>[4x]HMSVNKVTCLVCRKGDNDEFLLLCDGCDRGCHIYCHRPKMEAVPEGDWFCTVCLAQQV;>ARTKQTARKS[2x]

The plant homeodomain (PHD) finger is one of the largest families of epigenetic reader domains present in chromatin-related proteins, with over 170 PHD fingers identified in the human genome. Members of the BAZ family of proteins, which includes BAZ1A, also known as Acf1, BAZ1B, also known as Wstf, BAZ2A, also known as TIP5 (TTF-I/interacting protein 5), and BAZ2B, are all characterized by the presence of a PHD–BRD tandem module at their C-terminus. BAZ2A binds to the ATPase SNF2h (sucrose nonfermenting protein 2 homolog) to form the chromatin remodeling complex NoRC (nucleolar remodeling complex), which plays an essential role in silencing ribosomal DNA (rDNA) genes. Experiments performed with truncated versions of BAZ2A showed that the PHD–BRD module plays an important role in NoRC formation, with the PHD domain being required for interaction with the nucleosome to trigger transcriptional silencing of rDNA.

The peptide residues A1-K4 form an antiparallel β-sheet with the first β-strand of BAZ2A PHD, anchored by backbone hydrogen bonds with residues D1688, L1692, L1693, P1714 and G1716. However, starting from K4, the peptide adopts a helical fold that extends at least until R8, forming a complete loop of an α-helix. The canonical intrapeptide i to i + 4 backbone hydrogen bonds stabilize the helix loop i.e. T3 to A7 and K4 to R8. Two additional side chain-to-backbone intramolecular hydrogen bonds are formed, one between the T3 hydroxyl group and the amino group of T6, and a second one between the hydroxyl group of T6 and the amino group of R2. There is no interpretable density for K9 and S10, suggesting that these are disordered. Inspection of the binding pockets in each of the four chains of the asymmetric unit reveals that the histone-binding sites of chains A and D are both occupied by H3 10-mer and are free from crystal contacts that might interfere with or modulate the secondary structure of the peptide itself. Conversely, crystal packing occludes the binding sites of chains B and C and no peptide is found bound to these protomers. However strikingly, the structure shows no direct interactions between residues T6-S10 and the protein, besides a potential long-range hydrophobic contact between the A7 methyl group and the L1693 side chain. The 310 helix of BAZ2A PHD blocks H3 from binding in such an extended conformation, forcing it to fold back.> YLDHGLGAPAPYPDPLEPRREVCEL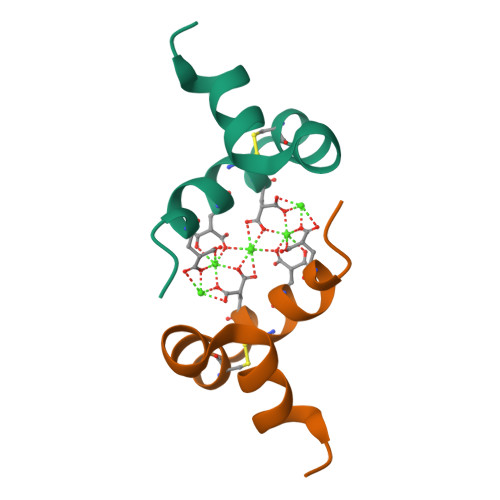NPDCDELADHIGFQEAYRRFYGIA> QCDNFPQMLRDLRDAFSRVKTFFQTKDEVDNLLLKESLLEDFKGYLGCQALSEMIQFYLEEVMPQAEN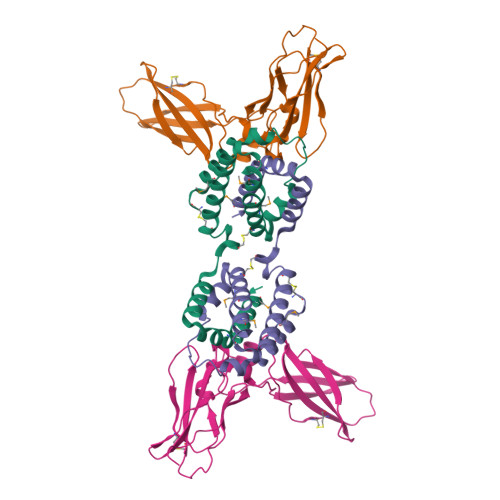QDPEIKDHVNSLGENLKTLRLRLRRCHRFLPCENKSKAVEQIKNAFNKLQEKGIYKAMSEFDIFINYIEAYMTIKAR;> HGTELPSPPSVWFEAEFFHHILHWTPIPQQSESTCYEVALLRYGIESWNSISQCSQTLSYDLTAVTLDLYHSNGYRARVRAVDGSRHSQWTVTNTRFSVDEVTLTVGSVNLEIHNGFILGKIQLPRPKMAPAQDTYESIFSHFREYEIAIRKVPGQFTFTHKKVKHEQFSLLTSGEVGEFCVQVKPSVASRSNKGMWSKEECISLTRQYFTVTN>[2x]SVPQISQPHFLLDGLSSQPLFNDIAAGIPSITAYSKNGLKIEFTFERSNTNPSVTVITIQASNSTELDM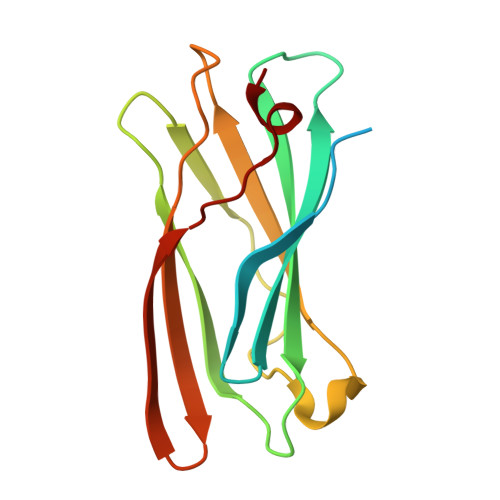TDFVFQAAVPKTFQLQLLSPSSSIVPAFNTGTITQVIKVLNPQKQQLRMRIKLTYNHKGSAMQDLAEVNNFPPQSWQ> 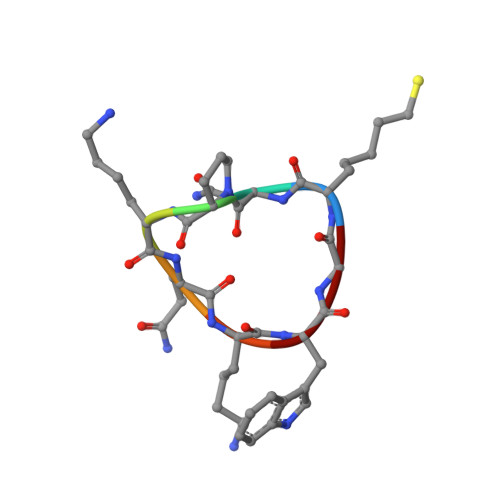XNPKQKWG> HHHHMVDAAVAEKLEAGFQKLQEATNCKSLLKKHLTREIFDKIKDLKTSFGSTLLDVIQSGVENLDSGFGVYAPDAEAYSVFNDLFEPMICDYHTGFKPGDAHPPRDFGDLETFGNLDPEGAFIVSTRVRCGRSLAGYAFNPCLTEANYKEMEEKVVASLSSLEGELKGTYYPLTGMTKEVQTQLIQDRFLFKEGDRFLQAANACRYWPTGRGIYHNDAKTFLVWCNEEDHLRIISMQKGGDLKAVYARLVNAINEIEKRIPFSHHDKYGFLTFCPTNLGTTIRASVHIALPKLAADLAKLEEAAGKFNLQVRGTA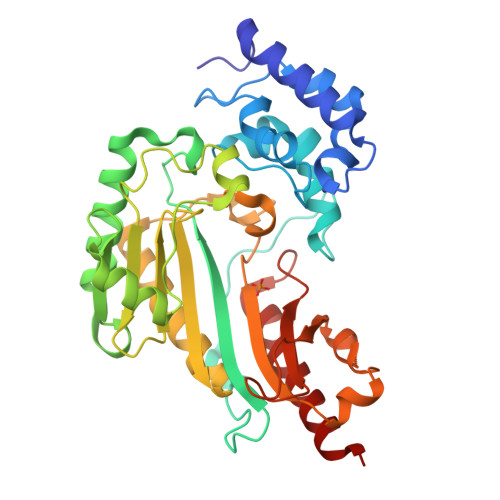GEHTEAEGGVYDISNKRRMGLTEYQAVKEMYDGLQELIRMEKEAA The type IV pilus is a diverse molecular machine capable of conferring a variety of functions and is produced by a wide range of bacterial species. The T4P is a filamentous polymer made of type IV pilins, the individual protein monomer (PilA), that is polymerized by several chaperones and minor pilins to form fibers that can extend micrometres in length with an outer diameter of ∼5–8 nm. The general architecture of the type IV pilin protein is an extended N-terminal α-helix connected by an α–β loop to a four- to seven-stranded β-sheet, termed the head domain, which packs onto one half of the α-helix. The C-terminal globular head domain faces the exterior of the assembled pilus, and in P. aeruginosa pilin proteins it features a conserved disulfide-bonded loop region that is responsible for cellular and surface adhesion termed the D-region.

Here, the 1.3 Å resolution crystal structure of the N-terminally truncated type IV pilin from P. aeruginosa strain P1 (ΔP1) is reported, the first structure of its phylogenetically linked group (group I) to be discussed in the literature. The α–β loop immediately follows the amphipathic α1-C helix, and the receptor-binding D-region with the conserved disulfide bond to the last strand of the β-meander is present. In the final model, all residues except the N-terminal side chain (Ile25) were observed, and 216 water molecules and a cacodylic acid molecule could be modeled in the electron density. The cacodylic acid also makes hydrogen bonds which stabilize the α–β loop and the α1-C helix as its O atoms hydrogen-bond to the side chain of Thr73 (2.46 Å) and water 17 (2.94 Å, B factor of 20.59 Å2), which connects to the helix through a hydrogen bond to the side chain of Glu39 (2.75 Å). The conserved disulfide bond is formed by Cys127 in the fourth β-sheet and Cys145; however, Cys127 is observed to have electron density representative of an unbonded cysteine (∼20% occupancy), which is likely to be due to radiation-induced breakage of the disulfide bond. Asn91 and Lys92 have particularly high B factors for this region (17.5 and 18.9 Å2, respectively), which is especially interesting as the residue which differs between P1 and 1244 is Lys92 (Gln in 1244), indicating that this flexible region may be of importance in the specificity and recognition of P. aeruginosa group Ia pili. Regarding the positioning of the monomers, there are clashes that occur between the α–β loop residues Pro63–Thr66 of one monomer and the D-loop residues Pro138–Ala141 of the other monomer; these regions are not pronounced in ΔK122.

> ISEFARTQVTRAVSEVSALKTAAESAILEGKEIVSSATPKDTQYDIGFTESTLLDGSGKSQIQVTDNKDGTVELVATLGKSSGSAIKGAVITVSRKNDGVWNCKITKTPTAWKPNYAPANCPKS> MRRFAAGCLALALLVLPFVLTGARAAEDESEKEIERYRQMIEDPMANPGFLNVDRGEVLWSEPRGTRNVSLETCDLGEGPGKLEGAYAHLPRYFADTGKVMDLEQRLLWCMETIQGRDTKPLVAKPFSGPGRTSDMEDLVAFIANKSDGVKIKVALATPQEKEMYAIGEALFFRRSSINDFSCSTCHGAAGKRIRLQALPQLDVPGKDAQLTMATWPTYRVSQSALRTM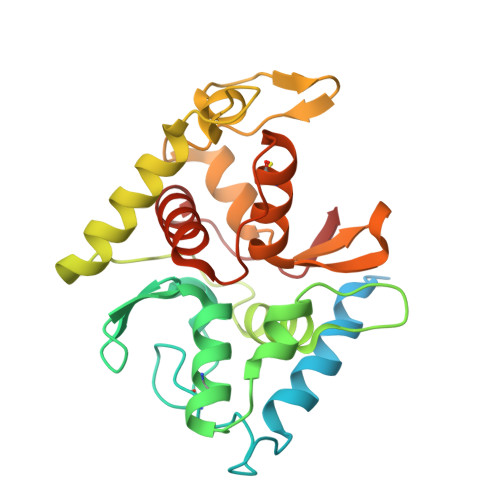QHRMWDCYRQMRMPAPDYASEAVTALTLYLTKQAEGGELKVPSIKR(S)-Methylmalonyl-Coenzyme A | C25 H40 N7 O19 P3 S | 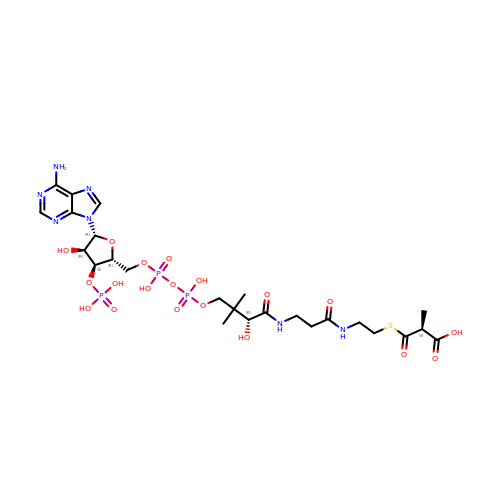MZFOKIKEPGUZEN-IBNUZSNCSA-N> MSHHHHHHSGLVPRGSMAWHLGIRSQSRPNDIMAEVCRAIKQLDYEWKVVNPYYLRVRRKNPVTSTFSKMSLQLYQVDSRTYLLDFRSIDDEITEAKSGTATPQRSGSISNYRSCQRSDSDAEAQGKPSEVSLTSSVTSLDSSPVDVAPRPGSHTIEFFEMCANLIKNSCTVN;> MGPYGQEMYAFRSEERFKSPPILPPHLLQVILNKDTNISCDPALLPEPNHVMLNHLYALSIKDSVMVLSATHRYKKKYVTTLLYKPI;> MESVAAESAPAPENEHSQETPESNSSVYTTFMKSHRCYDLIPTSSKLVVFDTSLQVKKAFFALVTNGVRAAPLWDSKKQSFVGMLTITDFINILHRYYKSALVQIYELEEHKIETWREVYLQDSFKPLVCISPNASLFDAVSSLIRNKIHRLPVIDPESGNTLYILTHKRILKFLKLFITEFPKPEFMSKSLEELQIGTYANIAMVRTTTPVYVALGIFVQHRV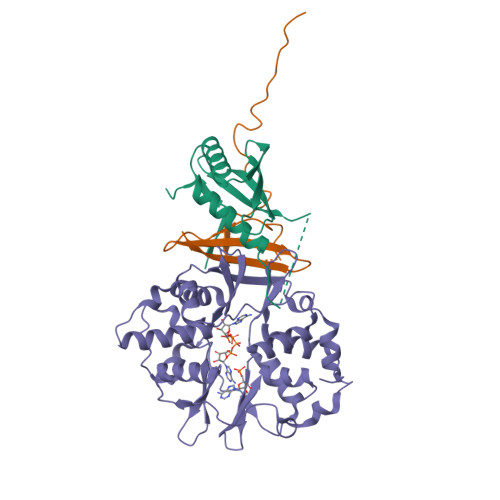SALPVVDEKGRVVDIYSKFDVINLAAEKTYNNLDVSVTKALQHRSHYFEGVLKCYLHETLEAIINRLVEAEVHRLVVVDEHDVVKGIVSLSDILQALVLTGGEKKP> MKQYLELMQKVLDEGTQKNDRTGTGTLSIFGHQMRFNLQDGFPLVTTKRCHLRSIIHELLWFLQGDTNIAYLHENNVTIWDEWADENGDLGPVYGKQ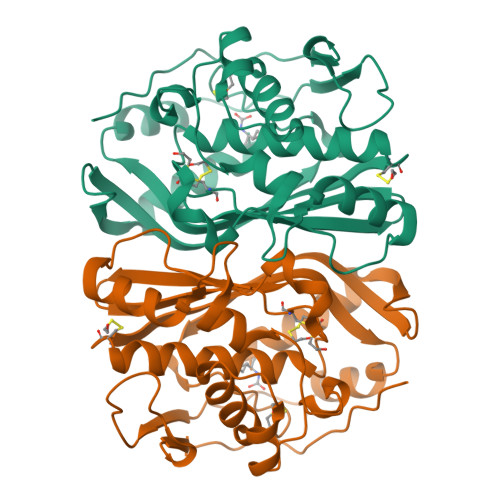WRAWPTPDGRHIDQITTVLNQLKNDPDSRRIIVSAWNVGELDKMALAPCHAFFQFYVADGKLSCQLYQRCCDVFLGLPFNIASYALLVHMMAQQCDLEVGDFVWTGGDTHLYSNHMDQTHLQLSREPRPLPKLIIKRKPESIFDYRFEDFEIEGYDPHPGIKAPVAI>GQEIRPMPADSAYGVVHISVCNMRDEGKFTSGMSTQALLGMPVKVLQYTGWYEIQTPDDYTGWVHRMVITPMSKEKYDEWNRAEKIVVTSHYGFTYEKPDDDSQTVSDVVAGNR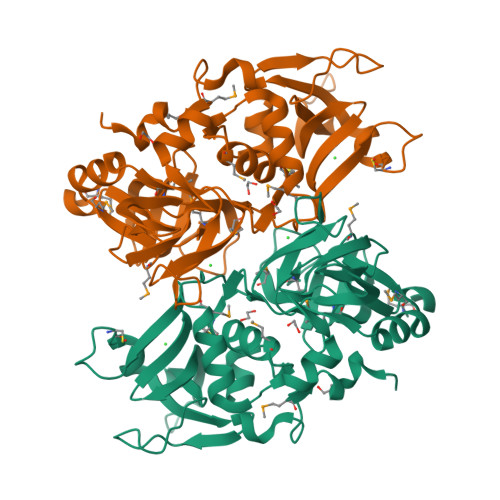LKWEGSKGHFYKVSYPDGRQAYISRHISQPESKWRASLKQDAESIIKTAYTMIGIPYLWAGTSSKGVDCSGLVRTVLFMHDIIIPRDASQQAYVGERIEIAPDFSNVQRGDLVFFGRKATADRKEGISHVGIYLGNKRFIHALGDVHISSFDPEDECYDEFNTGRLLFATRFLPYINKEKGMNTTDHNLYYLHH[2x]>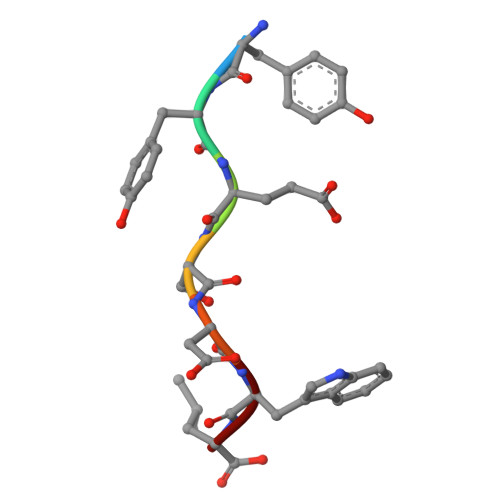 YYESDWL Rspo (R-spondin, also roof plate-specific spondin) proteins are evolutionarily conserved from fish to humans and have well-documented roles in a broad range of developmental and physiological processes resulting from enhancement of canonical and non-canonical Wnt signalling. ZNRF3/RNF43 specifically targets these Wnt receptors for ubiquitination and turnover, hence reducing Wnt signalling responses. Direct extracellular interaction with Rspo proteins inhibits ZNRF3/RNF43 activity. Here we report a molecular level analysis of the ZNRF3/RNF43 ectodomain structure and its interactions with Rspo proteins.

Sequence analyses suggest a putative domain structure for the Rspo proteins comprising two furin-like cysteine-rich regions (Fu domains) plus a thrombospondin type 1 repeat domain3. We therefore engineered constructs to express the region spanning the two Fu domains of Rspo2 proteins from several species. By using a combination of heavy atom and molecular-replacement-based phasing strategies, we determined multiple crystal structures for Xenopus (x) Rspo2Fu1–Fu2 (highest resolution 2.2 Å), xZNRF3ecto, zebrafish (z) ZNRF3ecto and mouse (m) ZNRF3ecto, (highest resolutions 2.4, 1.6 and 2.0 Å, respectively), plus complexes comprising xZNRF3ecto–xRspo2Fu1–Fu2, mZNRF3ecto–mRspo2Fu1–Fu2, mZNRF3ecto–xRspo2Fu1–Fu2 and xRNF4F3ecto–xRspo2Fu1–Fu2 (at 2.1, 2.8, 2.4 and 2.7 Å, respectively). In the crystal structure of the isolated RspoFu1–Fu2 protein the two Fu domains arrange sequentially to form a ladder-like structure of β-hairpins. Each Fu domain comprises three β-hairpins rigidified by four disulphide bridges, similar to the cysteine-rich regions found in members of the epidermal growth factor receptor family. The connection between the Fu domains shows considerable rotational freedom, allowing a 50°–60° variation in the relative interdomain orientation. The N terminal of the two domains, Fu1, is distinguished by the extension of the second β-hairpin. This prominent loop presents a solvent exposed methionine (M68) at its tip, which we term the ‘Met-finger’.

>[8x]ETGGTNPICKGCLSCSKDNGCLRCQPKLFFYLRREGMRQYGECLQSCPPGYYGVRGPDMNRCSRCRIENCDSCFSRDFCIKCKSGFYSHKGQCFEECPEGFAPLDDTMVCVDGTKHHHHHH> GHMTQGQTPPEELSADPSPETGALAPAKARMRELATAYARRLPGLDTHSLMSGLDATLTFMPMGDRDGAYDPEHRVVLINSRVRPERQRFTLAHEISHALLLGDDDLLSDLHDAYEGERLEQVIETLCNVGAAAILMPETLIDELLARFGPSGRALAELARRADVSASSALYALAERTSVPVLYAVCAVSRLEAESGEERLPEKALTVRASAGSPGVKYSLRPGTLIPDDHPVAVALETRLPITQESYVPFRSGRRMPAYVDAFPERQRVLVSFALLPKATKGGEQDESGV

A protease-based derepression mechanism in response to DNA damage was characterized in Deinococcus, which is controlled by the specific cleavage of repressor DdrO by metallopeptidase PprI (also called IrrE). In coordination with the transcriptional repressor DdrO, which binds to the radiation/desiccation response motif (RDRM)-containing promoters upstream of DDR genes, the specific cleavage of DdrO by PprI induces the expression of DDR proteins following DNA damage. DG-PprI, which is comprised of 9 α-helices and 8 β-strands, contains three domains: an N-terminal zinc peptidase-like domain (residues 19-135), a helix-turn-helix domain (HTH domain, residues 136-176), and a C-terminal GAF-like domain (residues 177-277). Single-stranded DNA (ssDNA) physically bound to Deinococcus geothermalis PprI (termed DG-PprI for brevity) and stimulated its protease activity in a length-dependent manner.

We first determined the crystal structure of full-length DG-PprI at the resolution of 2.8 Å (Rwork/Rfree=0.247/0.284) in the presence of Mn2+, which is effective for its protease activity. Despite weak electron density in apo structure, a catalytic manganese ion (Mn2+) lies in the active site of DG-PprI, coordinated by the conserved HEXXH motif (HEISH in DG-PprI) of the N-terminal zinc peptidase-like domain. Interestingly, strong electron density was observed on top of the HTH domain of DG-PprI, which is interpreted as the sulfate ion present at 1.7 M in the crystallization reservoir solution. This sulfate ion is located at the positively charged cavity formed by residues from the zinc peptidase-like domain (Arg85) and GAF-like domain (Arg207 and Arg267). Given that HTH motifs are commonly found in DNA binding proteins and sulfate might mimic the chemistry of a phosphate group, we further investigated the possible DNA binding capability of DG-PprI. Moreover, arginine residues forming the sulfate-binding cavity are required for ssDNA binding. While the double mutants (R85A/R207A and R207A/R267A) showed smeared shifted bands, the triple mutant R85A/R207A/R267A totally abolished the ssDNA binding of DG-PprI. In the absence of ssDNA, PprI exhibited limited protease activity in vitro and adopted an open cleavage site with side-by-side dimer formation.> GSHMDVAGLTDCGLIR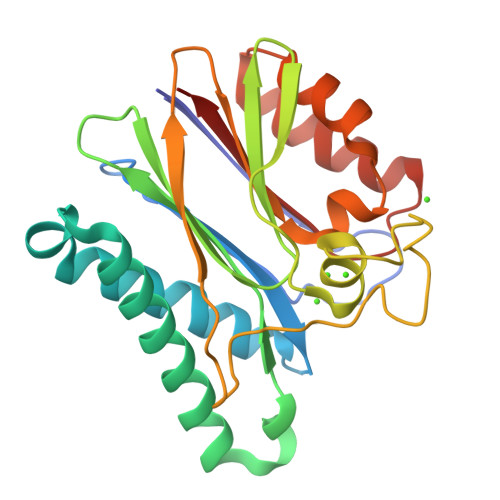KSNQDAFYIDEKHQRFFIVADGMGGHAGGEEASRLAVDHIRQYLETHLEDLQHDPVTLLRQAFLAANHAIVEQQRQNSARADMGTTAVVILLDEKGDRAWCAHVGDSRIYRWRKDQLQQITSDHTWIAQAVQLGSLTIEQARQHPWRHVLSQCLGREDLSQIDIQPIDLEPGDRLLLCSDGLTEELTDDVISIYLSEPNVQKAAAALVDAAKTHGGRDNVTVVVISV> SNIDGMKLYLQHCKTCHGVDG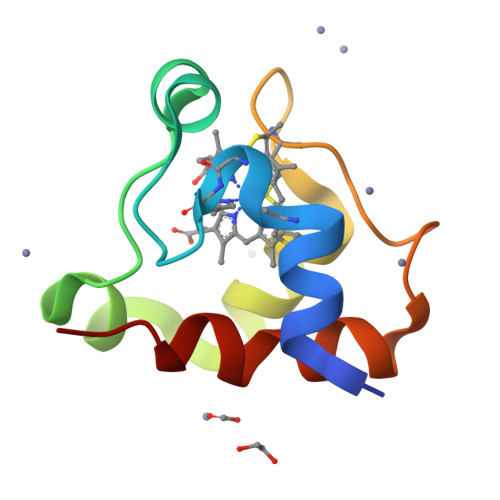NPTDLGEGLGARKFADAEWQAKTSDERIIEQINEGTPEMMMPFKEKLTPEEVKALVPVVRGFKK> TCGGCGCCGA

Here, we report two crystal structures of Δ-[Ru(phen)2(dppz)]2+ in the presence of an oligonucleotide decamer that may help with interpreting the photophysics of the compound when bound to DNA in solution. The structure shows Δ-[Ru(phen)2(dppz)]2+ bound to d(TCGGCGCCGA)2 by two distinctly different binding modes. The complex binds into the minor groove and end-caps the duplex at both ends, with both T1 and A10 flipped out.

The two structures presented here only differ, in gross structural terms, in the presence of Ba2+ or cobalt hexammine at the semi-intercalation site. In structure 1, which contained BaCl2 in the crystallisation condition, Ba2+ coordinates to the guanine bases at the N7 position. We have previously reported this binding mode in a number of our structures with the Λ enantiomer of [Ru(phen)2(dppz)]2+ and [Ru(TAP)2(dppz)]2+ and derivatives. When Ba2+ is bound to G3 and G4 (structure 1), the twist at the central step is 32°. Steps G4C5:G6C7 and G3G4:C7C8 have a twist of 33° and 21°, respectively. The Ba2+, acting as an anchor point, reduces the twist at the semi-intercalation site by 2°, when compared to the cobalt hexammine bound form. This seemingly small difference results in a reduced twist at the G4C5:G6C7 step which must be corrected by an increased twist at the central step. At the central step the roll angle in both structures is <6° and therefore the DNA structure is not significantly kinked. The overall structure of the DNA duplex, based on the predominant sugar pucker, is that of an A/B hybrid.>[4x]MSFEGARLSMRSRRNGTMGSTRTLYSSVSRSTDVSYSDSDLVNFIQANFKKRECVFFTRDSKAMENICKCGYAQSQHIEGTQINQNEKWNYKKHTKEFPTDAFGDIQFETLGKKGKYLRLSCDTDSETLYELLTQHWHLKTPNLVISVTGGAKNFALKPRMRKIFSRLIYIAQSKGAWILTGGTHYGLMKYIGEVVRDNTISRNSEENIVAIGIAAWGMVSNRDTLIRSCDDEGHFSAQYIMDDFTRDPLYILDNNHTHLLLVDNGCHGHPTVEAKLRNQLEKYISERTSQDSNYGGKIPIVCFAQGGGRETLKAINTSVKSKIPCVVVEGSGQIADVIASLVEVEDVLTSSMVKEKLVRFLPRTVSRLPEEEIESWIKWLKEILESSHLLTVIKMEEAGDEIVSNAISYALYKAFSTNEQDKDNWNGQLKLLLEWNQLDLASDEIFTNDRRWESADLQEVMFTALIKDRPKFVRLFLENGLNLQKFLTNEVLTELFSTHFSTLVYRNLQIAKNSYNDALLTFVWKLVANFRRSFWKEDRSSREDLDVELHDASLTTRHPLQALFIWAILQNKKELSKVIWEQTKGCTLAALGASKLLKTLAKVKNDINAAGESEELANEYETRAVELFTECYSNDEDLAEQLLVYSCEAWGGSNCLELAVEATDQHFIAQPGVQNFLSKQWYGEISRDTKNWKIILCLFIIPLVGCGLVSFRKKPIDKHKKLLWYYVA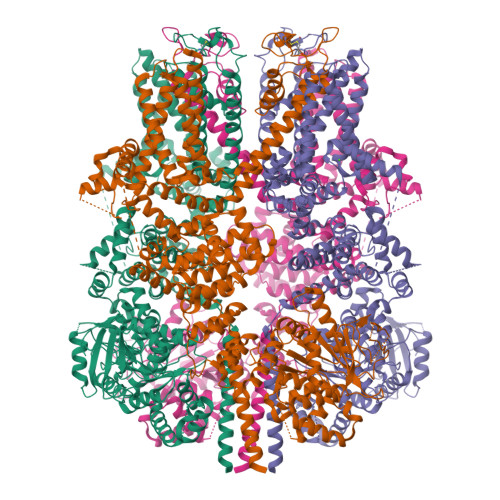FFTSPFVVFSWNVVFYIAFLLLFAYVLLMDFHSVPHTPELILYALVFVLFCDEVRQWYMNGVNYFTDLWNVMDTLGLFYFIAGIVFRLHSSNKSSLYSGRVIFCLDYIIFTLRLIHIFTVSRNLGPKIIMLQRMLIDVFFFLFLFAVWMVAFGVARQGILRQNEQRWRWIFRSVIYEPYLAMFGQVPSDVDSTTYDFSHCTFSGNESKPLCVELDEHNLPRFPEWITIPLVCIYMLSTNILLVNLLVAMFGYTVGIVQENNDQVWKFQRYFLVQEYCNRLNIPFPFVVFAYFYMVVKKCFKCCCKEKNMESNACCFRNEDNETLAWEGVMKENYLVKINTKANDNSEEMRHRFRQLDSKLNDLKSLLKEIANNIKLEGGSSGGWSHPQFEK> MNTFFLTPAAAAARRVAVSFFARSSASGFPQHRVALRPF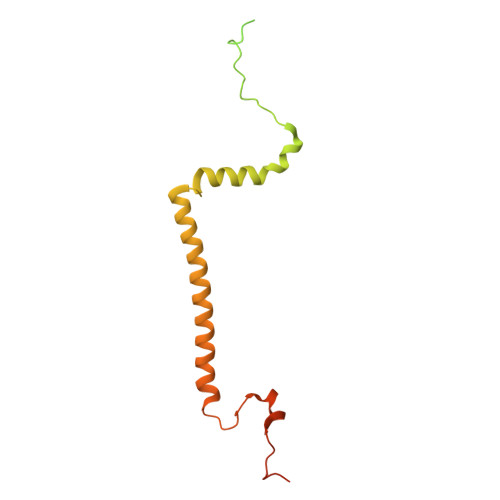PSQRPAERAHNLAKSQTLRSVKAHGRQSGKKEQSTESGGRRGFRAAVGAGTGCMLAASPMLFTDYDNTASPKSELIFMAGNALGYCTERFFENEYGQSIFMFALGLAYLAMLGHEGKIHGAVWRMKHLFATNFKMVGHPRYAYALPKNPLLQDAAPTKTGSTSAKK> MQGSVTEFLKPRLVDIEQVSSTHAKVTLEPLERGFGHTLGNALRRILLSSMPGCAVTEVEIDGVLHEYSTKEGVQEDILEILLNLKGLAVRVQGKDEVILTLNKSGIGPVTAADITHDGDVEIVKPQHVICHLTDE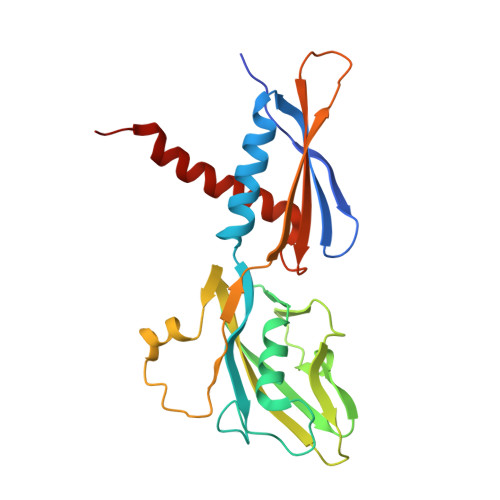NASISMRIKVQRGRGYVPASTRIHSEEDERPIGRLLVDACYSPVERIAYNVEAARVEQRTDLDKLVIEMETNGTIDPEEAIRRAATILAEQLEAFVDLRD> KEITNALETWGALGQDINLDIPSFQMSDDIDDIKWEKTSDKK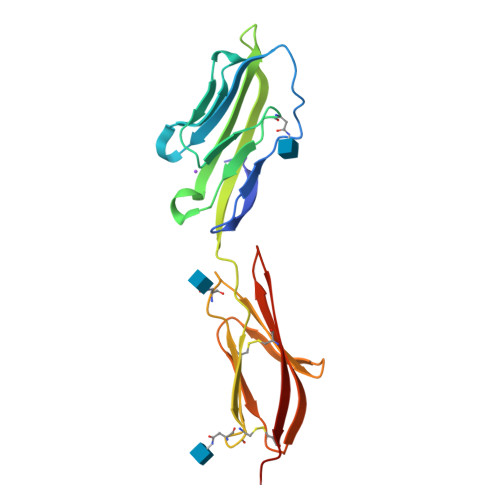KIAQFRKEKETFKEKDTYKLFKNGTLKIKHLKTDDQDIYKVSIYDTKGKNVLEKIFDLKIQERVSKPKISWTCINTTLTCEVMNGTDPELNLYQDGKHLKLSQRVITHKWTTSLSAKFKCTAGNKVSKESSVEPVSCPEK>MRVSLRSITSLLAAATAAVLAAPAAETLDRRAALPNPYDDPFYTTPSNIGTFAKGQVIQSRKVPTDIGNANNAASFQLQYRTTNTQNEAVADVATVWIPAKPASPPKIFSYQVYEDATALDCAPSYSYLTGLDQPNKVTAVLDTPIIIGWALQQGYYVVSSDHEGFKAAFIAGYEEGMAILDGIRALKNYQNLPSDSKVALEGYSGGAHATVWATSLAESYAPELNIVGASHGGTPVSAKDTFTFLNGGPFAGFALAGVSGLSLAHPDMESFIEARLNAKGQRTLKQIRGRGFCLPQVVLTYPFLNVFSLVNDTNLLNEAPIASILKQETVVQAEASYTVSVPKFPRFIWHAIPDEIVPYQPAATYVKEQCAKGANINFSPYPIAEHLTAEIFGLVPSLWFIKQAFDGT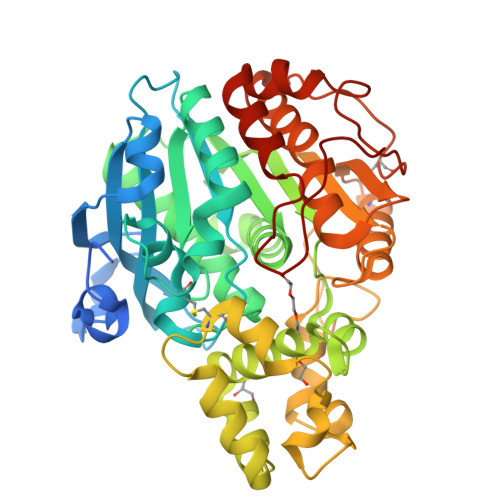TPKVICGTPIPAIAGITTPSADQVLGSDLANQLRSLDGKQSAFGKPFGPITPP[2x]>MASAANAGQLGNLPGVTSMGMGYDVNGLYASPESLLGQPLFDFGGELDSIEIEGRSYTFPRSMHVHTYFHSDFKQDVSKEIEEYREKMSQHVGVSGRYKLFSASLSVDFTTTDQQLTEITYSSTREAHVLWYISLPGAATLRSMLRRDFRDDLNNPNMPAMELFKRYGPYYISEAAVGGRLDYSAASKTLKMDSSQSLSTTAEMSYKALVGEIKIEHGSEMEKQVNSFRSNSTIRLTATGGKPGMTDRILHGPDSQQAFSQWAESLLDYATLMDFSTESLQPIWALADKPERRVELEDAFPEFMKQSQQSIPKVDKVLLMDARPPMVKAGEDSGSGASEDLAVFNPSTSNGYKMVGQFGQRNHASVADGHAPIFKDLFDLGVLKAPVGWQRVWDDAGSGKSKDYACWRAIPPQGYRALGDVMMLATSGYNPPNLPDYVCVHQSLCADVQTLQNRVWWDKGTGARKDVSLWQPGAAGAVASSCFAGVPNYNNPPNSGDIERLRGSIACVKTSAIAS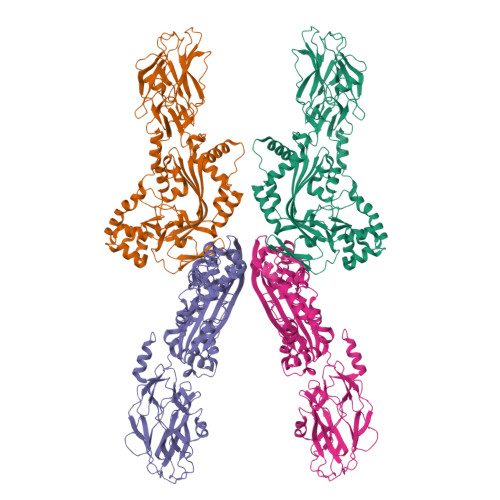MQEMKSMLSQHQGMEAMMSKL[4x]N-[4-(2-fluoropyridin-4-yl)thiophen-2-yl]-2-{3-[(methylsulfonyl)amino]phenyl}acetamide 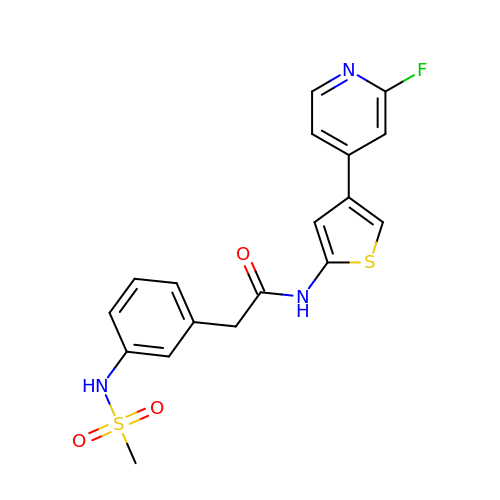| C18 H16 F N3 O3 S2 | IVWXFGRLNHCKNV-UHFFFAOYSA-N> HHHHHHGNMREIAPKEFVLDMGAGWNLGNAMDTYNSDETAWGNPLTTKAMIDEIAKMGFKTLRLPVTWKFHIGEGPDYLIEANWLDKVEAIANFALENEMYVIINIHHDETWIL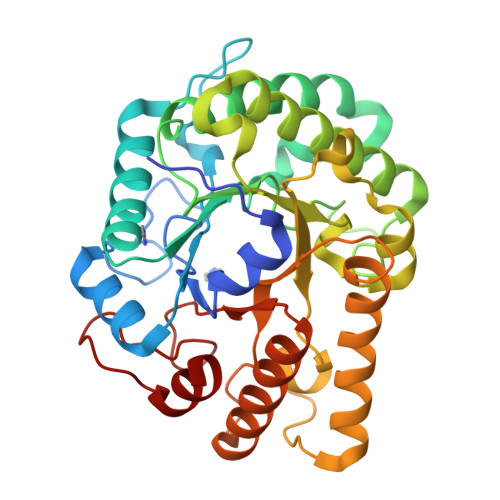PTYEKADEVKDELSKVWTQIANRFKTYGDYLIFETLNEPRHKGTPEEWKGGTQEGRDAVNQYHQVSVDAIRATGGNNAKRKIMVSTYAASTASNALNDYLVPNGDKNVIVSVHSYFPYQFCLDGTDSTWGTEADKTALLAELDKIRDKFIVEDNRAVVMGEWGSTFSDNPEDRLAHAEFYARACAERGICPIWWDNGNVDEFGIFNRNTLEWNYPEIAEAIVK> MADKVKSIQPGPIFYDVFLVYLRVIGTNLKDWCAPHGVTATNAKSAATGGWNGTKARALRQKMIDEVGEETF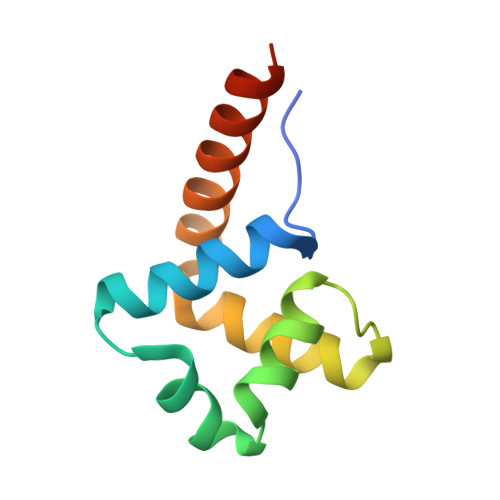LRLYTERLRREAALEHHHHHH>[2x]MEKLWLNSADSHVLEPDDLWERALPAALRDRAPRCVRDNGRETVYVDGQVVRRDPLDFADAMRPPGALDHHIRLKDLDDQGIWGEVVFPSRGLWTAVMTDPVLARECIKVYNDWLKSDFLSLSPRLVGAAMVSMLDTDDAVAELRRAADLGYQTVFLAATPPPGREFNMDVWEPLWAAAEEAGMTVSIHIGTGADTVV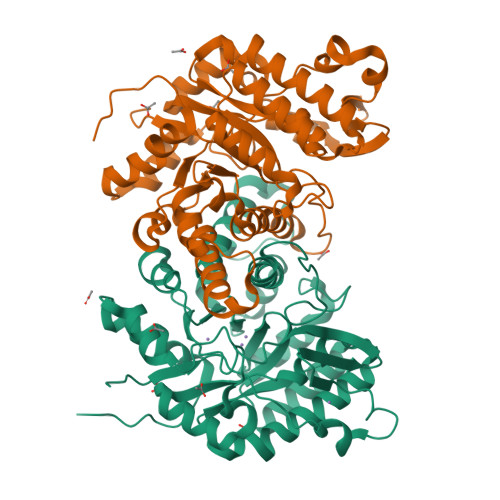ARGPGGAVINYVETLFPAQRAVAQLVASGALDRHPGLRVLIAEAGCAWVPALADRMDEAYRQHGMFVRPKLSMLPGELVRRQVYASFQHDETAIGAVTAMNYTNVLWGSDYPHLEGTFPRTQEVVTELFAGVDPEVRDLITRRNFTDLFTVPALPATV>MAEQVFQNFETLQLHAGYTPDPHTRSTAVPIYATSSYTFNDSAHGARLFGLKELGNIYSRLMNPTVDVFEKRIAALEGGIAAAATSSGQAAQFLTIATLAKAGDNIVASSHLYGGTYNQLNVLLPRFGIKTKFVRSGKLEDYAAAIDDQTRAIYVESMSNPDYVVPDFEGIAKIAHEHGIPLVVDNTLGAGGYYIRPIEHGADIVVHSATKWIGGHGTTIGGVIVDSGRFNWNKHSDRFPEMVEPSPSYHGLKYWEAFGPATFITRIRVEMLRDIGACLSPFSAQQLLLGIETLGLRAERHAQNTEKLSKYFESSPNVSWVLWPGSESHPTYSQAKKYLTRGFGAMLSIGVKGDASAGSKVVDGLKLVSNLANVGDAKSLAIHPWSTTHEQLSEDERLASGVTEDMIRISVGIEHVDDIIA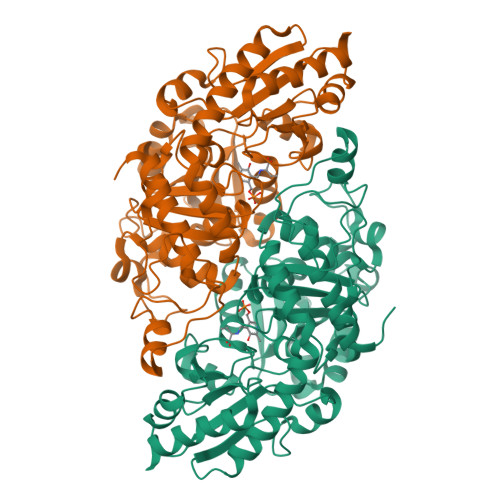DFEQSFQKAYGS[16x]2-{3-[(4-AMINO-2-METHYLPYRIMIDIN-5-YL)METHYL]-4-METHYL-2-OXO-2,3-DIHYDRO-1,3-THIAZOL-5-YL}ETHYL TRIHYDROGEN DIPHOSPHATE | C12 H18 N4 O8 P2 S | 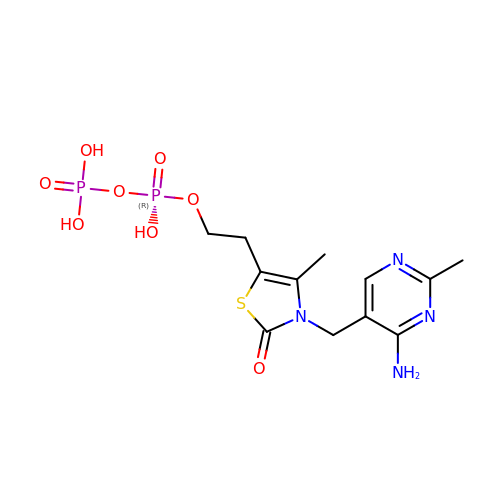ZGJUYGIRPQSCFA-UHFFFAOYSA-N>GRPFVEMYSEIPEIIHMTEGRELVIPCRVTSPNITVTLKKFPLDTLIPDGKRIIWDSRKGFIISNATY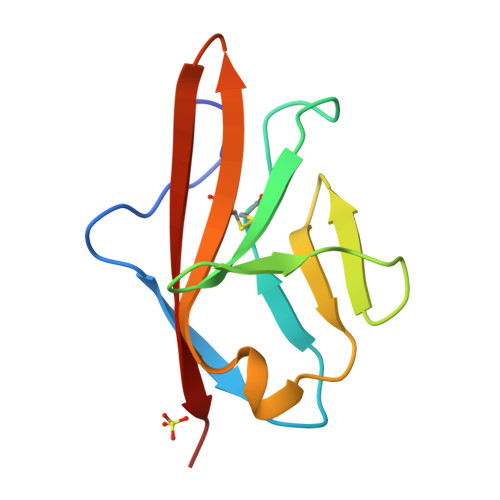KEIGLLTCEATVNGHLYKTNYLTHRQT[3x]> 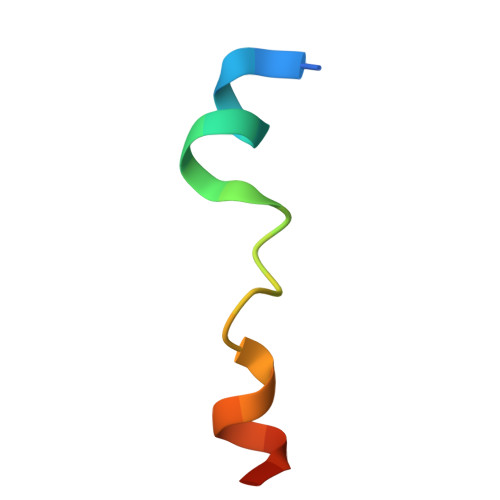GSHMFFEIFGTGEEYRYVLESDP> MGSDKIHHHHHHMKEIDELTIKEYGVDSRILMERAGISVVLAMEEELGNLSDYRFLVLCGGGNNGGDGFVVARNLLGVVKDVLVVFLGKKKTPDCEYNYGLYKKFGGKVVEQFEPSILNEFDVVVDAIFGTGLRGEITGEYAEIINLVNKSGKVVVSVDVPSGIDSNTGKVLRTAVKADLTVTFGVPKIGHILFPGRDLTGKLKVANIGHPVHLINSINRYVITREMVRSLLPERPRDSHKGTYGKVLIIAGSRLYSGAPVLSGMGS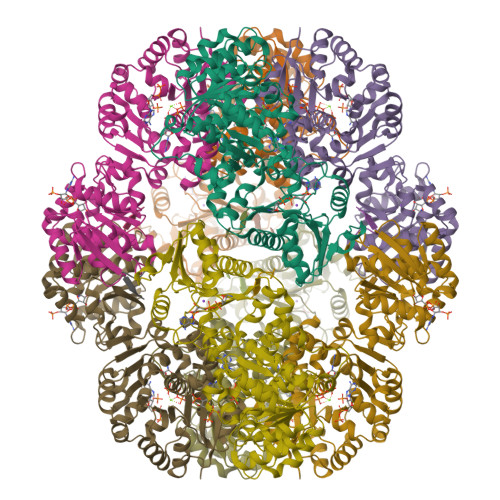LKVGTGLVKLAVPFPQNLIATSRFPELISVPIDTEKGFFSLQNLQECLELSKDVDVVAIGPGLGNNEHVREFVNEFLKTLEKPAVIDADAINVLDTSVLKERKSPAVLTPHPGEMARLVKKTVGDVKYNYELAEEFAKENDCVLVLKSATTIVTDGEKTLFNITGNTGLSKGGSGDVLTGMIAGFIAQGLSPLEASTVSVYLHGFAAELFEQDERGLTASELLRLIPEAIRRLKE;> PAWLFEA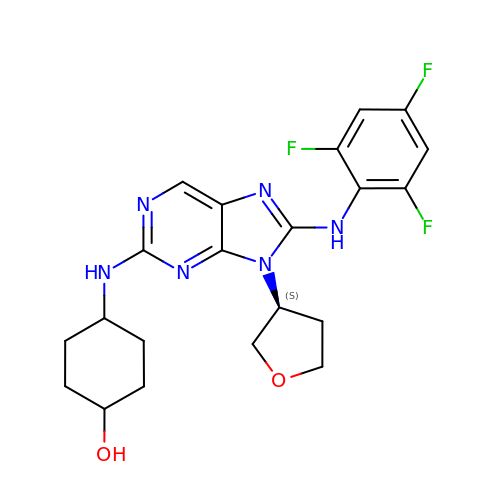trans-4-({9-[(3S)-tetrahydrofuran-3-yl]-8-[(2,4,6-trifluorophenyl)amino]-9H-purin-2-yl}amino)cyclohexanol | C21 H23 F3 N6 O2 | IBGLGMOPHJQDJB-IHRRRGAJSA-N>SMVCEVDPELTEKLRKFRFRKETDNAAIIMKVDKDRQMVVLEEEFQNISPEELKMELPERQPRFVVYSYKYVHDDGRVSYPLCFIFSSPVGCKPEQQMMYAGSKNRLVQTAELTKVFEIRTTDDLTEA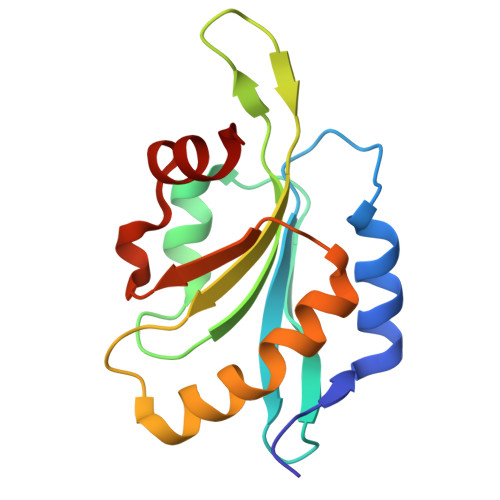WLQEKLSF[2x]>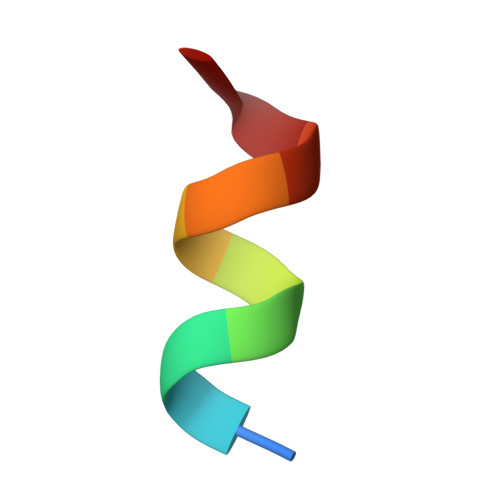 GAFQNLFQSV> LRMVETRTIVRF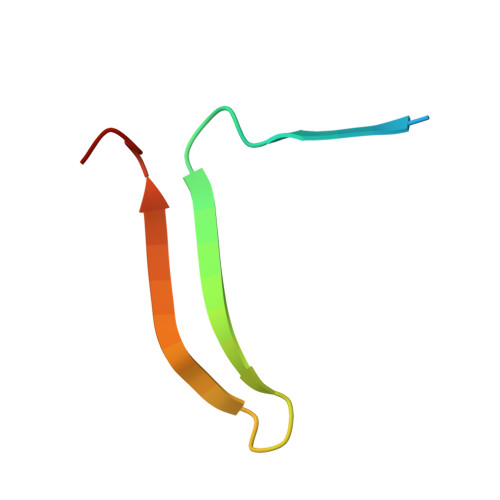NRPFLMIIVDHFTWSIFFMSKVTNPKQA> ACTKNAIAQTGFNKDKYFNGDVWYVTDYLDLEPDDVPKRYCAALAAGTASGKLKQALYHYDPKTQDTFYDVSELQVESLGKYTANFKKVDKNGNVKVAVTAGNYYTFTVMYADDSSALIHTCLHKGNKDLGDLYAVLNRNKDAAAGDKVKSA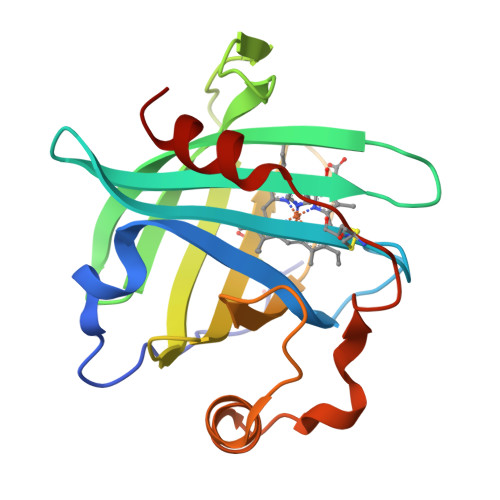VSAATLEFSKFISTKENNCAYDNDSLKSLLTK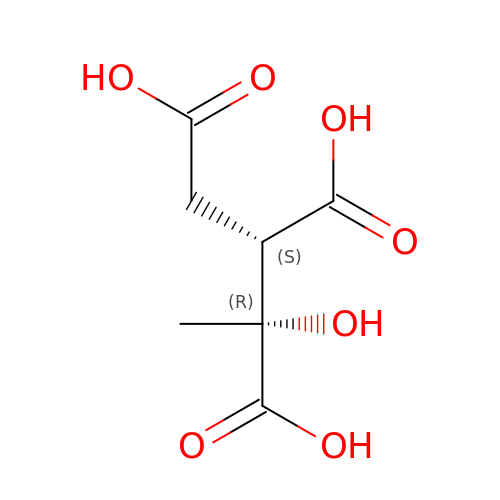ALPHA-METHYLISOCITRIC ACID | C7 H10 O7 | HHKPKXCSHMJWCF-WVBDSBKLSA-N>[4x]MTREDMEKRANEVANLLKTLSHPVRLMLVCTLVEGEFSVGELEQQIGIGQPTL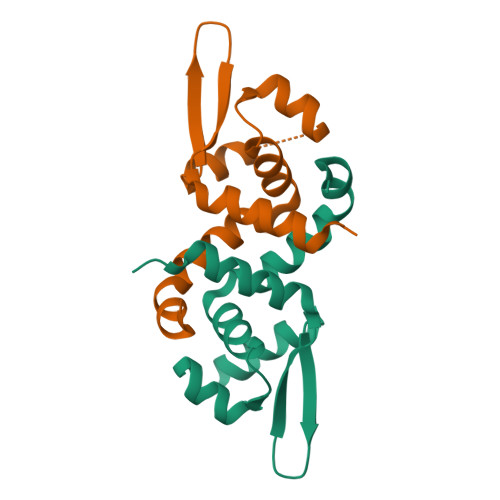SQQLGVLRESGIVETRRNIKQIFYRLTEAKAAQLVNALYTIFCAQEKQA3-fluoro-N-{(1R)-1-[(3P)-3-(1H-imidazol-1-yl)phenyl]ethyl}propan-1-amine 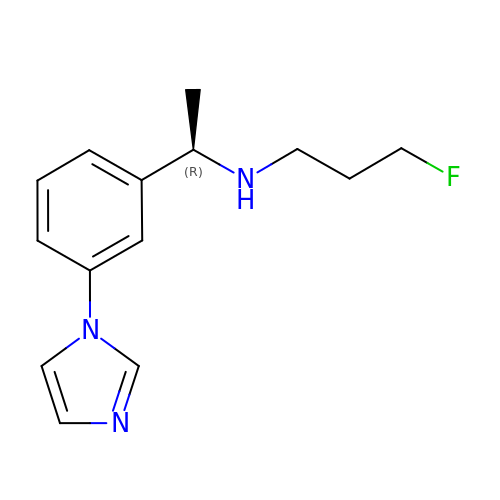| C14 H18 F N3 | FEBIPSXCUUTCKH-GFCCVEGCSA-N> SAELRPFICVNEKDHLPSLDPQADAWYRE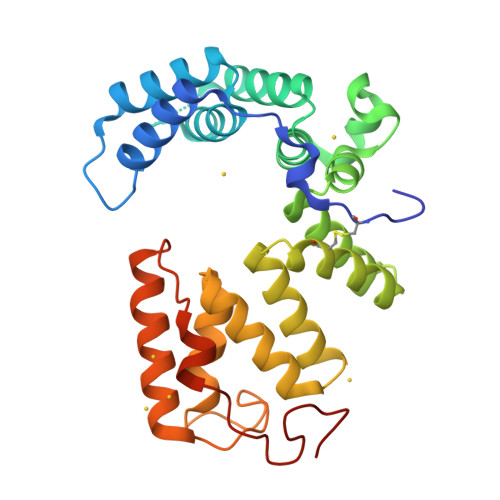AVALAKPDTLRPWDRIVDLYSKAVERGHWKAMHNLASLYRTGWPGGVEKDTQKALDLYQKMIDLKVPQGFYDMAAMIGNRAGVKNPATDGLTFLDKAASLGNPPALTELGRLYIYVAGQDELGLKYTNCAAGQGYAPANYELAMYYRLVAHNYPKAAGYYLLAASQGNDDAAFFMSGVFDKTSPDVDRMWYAPDEKLHKLYDGIYDQLAADPDLRFPNLIKDHPLPPHPTQGYDADRPDWKPGQ2-AMINO-6-HYDROXYMETHYL-7,8-DIHYDRO-3H-PTERIDIN-4-ONE 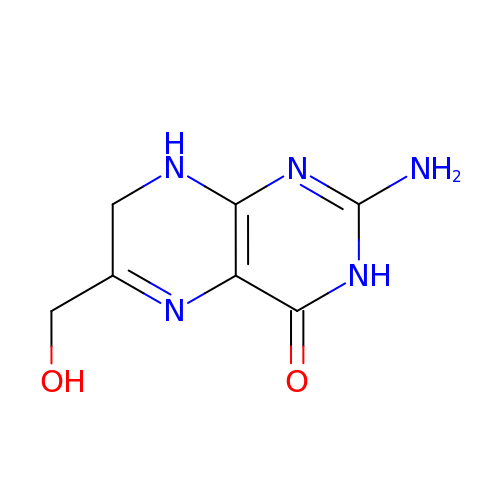| C7 H9 N5 O2 | CQQNNQTXUGLUEV-UHFFFAOYSA-N The replicative DNA polymerase from the hyperthermophilic archaeon Pyrococcus furiosus (Pfu) is a member of that polB family and is used extensively in biotechnology applications including high-fidelity PCR. We had previously used polymerase evolution by short patch compartmentalised self-replication (spCSR) to discover variants of Pfu with a dramatically enhanced ability to incorporate Cy3- and Cy5-labelled dCTP and replicate Cy-dye labelled DNA. The resulting variant E10, derived from an exonuclease-deficient version of Pfu polymerase (with mutations V93Q, D141A and E143A) and with additional mutations in the conserved A- (V337I, E399D, N400D, R407I) and C- active site sequence motifs (Y546H) was able to efficiently PCR DNA while completely replacing all dCTP on both strands with cyanine labelled dCTP (Cy3-dCTP or Cy5-dCTP) giving rise to highly-fluorescent products, termed Cy-DNA with applications in advanced microscopy applications. In an attempt to better understand the molecular basis for the altered substrate specificity of Pfu E10 polymerase and generally gain a better structural understanding of the primer-template duplex recognition in this class of DNA polymerases, we have solved the crystal structures of the apo Pfu-E10 and a Pfu-E10:DNA binary complex at 2.4 Å and 2.9 Å resolution respectively and compare them to previously obtained structures.

Pfu-E10 displays the domain structure characteristic of DNA polymerases, consisting of an N-terminal domain (residues 1–130), an exonuclease domain (131–326), a linker region (327–369), a palm domain (370–450 and 501–586), a fingers domain (451–500) and a thumb domain (587–775). The electron density is well defined for the N-terminal, exonuclease, linker, palm and fingers domains of both molecules in the crystallographic asymmetric unit, but some parts of the thumb domains are disordered. The final model for chain B is the most complete, but is missing amino acids 612–614, 669–675, 693–695 and 757–775. The two molecules (chains A and B) are very similar (rmsd of 0.8 Å for 690 alpha carbon atoms). There is a slight difference in the orientation of the thumb domain, which has a slightly more open conformation in chain B than chain A. This is likely to be due to the different crystal contacts in this region. The structure of apo Pfu-E10 is very similar to both these structures, with a superposition rmsd of 1.0 Å and 0.9 Å between Pfu-pol and Pfu-E10 (molecule A or B respectively, 685 residues aligned), and 1.0 Å rmsd between the Pfu-PCNA and Pfu:E10 Chain A (694 residues aligned) and 1.5 Å for Chain B (715 residues aligned). The greatest difference between the three models is in the thumb domain, especially in the region of residues 679–730.

>MILDVDYITEEGKPVIRLFKKENGKFKIEHDRTFRPYIYALLRDDSKIEEVKKITGERHGKIVRIVDVEKVEKKFLGKPITVWKLYLEHPQDQPTIREKVREHPAVVDIFEYDIPFAKRYLIDKGLIPMEGEEELKILAFAIATLYHEGEEFGKGPIIMISYADENEAKVITWKNIDLPYVEVVSSEREMIKRFLRIIREKDPDIIVTYNGDSFDFPYLAKRAEKLGIKLTIGRDGSEPKMQRIGDMTAVEVKGRIHFDLYHVITRTINLPTYTLEAVYEAIFGKPKEKVYADEIAKAWESGENLERVAKYSMEDAKATYELGKEFLPMEIQLSRLIGQPLWDVSRSSTGNLVEWFLLRKAYERNEVAPNKPSEEEYQRRLRESYTGGFVKEPEKGLWDDIVYLDFIALYPSIIITHNVSPDTLNLEGCKNYDIAPQVGHKFCKDIPGFIPSLLGHLLEERQKIKTKMKETQDPIEKILLDYRQKAIKLLANSFYGYYGYAKARWYCKECAESVTAWGRKYIELVWKELEEKFGFKVLYIDTDGLHATIPGGESEEIKKKALEFVKYINSKLPGLLELEYEGFYKRGFFVTKKRYAVIDEEGKVITRGLEIVRRDWSEIAKETQARVLETILKHGDVEEAVRIVKEVIQKLANYEIPPEKLAIYEQITRPLHEYKAIGPHVAVAKKLAAKGVKIKPGMVIGYIVLRGDGPISNRAILAEEYDPKKHKYDAEYYIENQVLPAVLRILEGFGYRKEDLRYQKTRQVGLTSWLNIKKS[2x]> GSASVTKLKNLKENSSNLIQLPLFINTTEAEFAAASVQRYELNMKA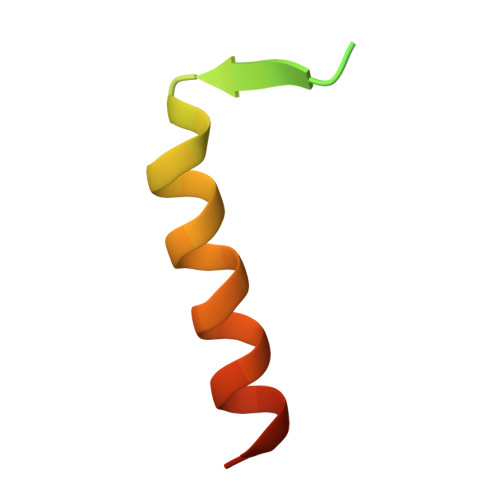LN>MPLSQEESTLIERATATINSIPISEDYSVASAALSSDGRIFTGVNVYHFTGGPCAQLVVLGTAAAAAAGNLTCIVAIGNENRGILSPCGRCRQVLLDLHPGIKAIVKDSDGQPTAVGIRELLPSGY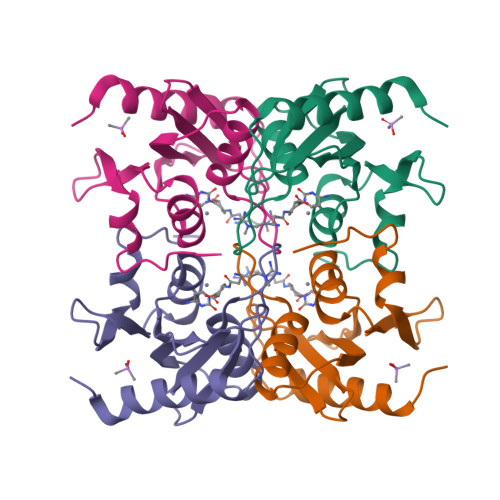VWEG[4x]(3E)-4-(1H-imidazol-4-yl)but-3-enoic acid | C7 H8 N2 O2 | 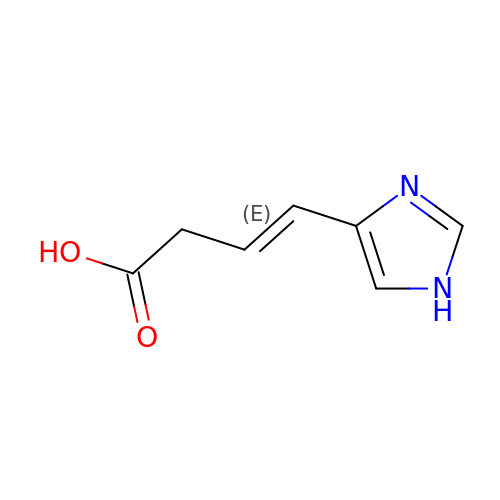KGQDUHSSIRUHKI-OWOJBTEDSA-N>GSHMLDGCTPWPAEFAVRYREAGYWTGETFSDFVTDRTRRFADRLAVVGAGQRWTYAELGERSAVLATGLARLGIAAGDRVVVQLPNIPELFEVVFALFRLGALPVYALPAHRAHEITHLCTTAQAKALIIPDRHAGFDYRTMAAQLRHAGTAPEHVVVVGEPGGFTPLAELRADRPDPGVFTRPEASDAAFLQLSGGTTGLPKLIPRTHDDYLYSVRASAEICALGTDTVYLAALPAVHNFPM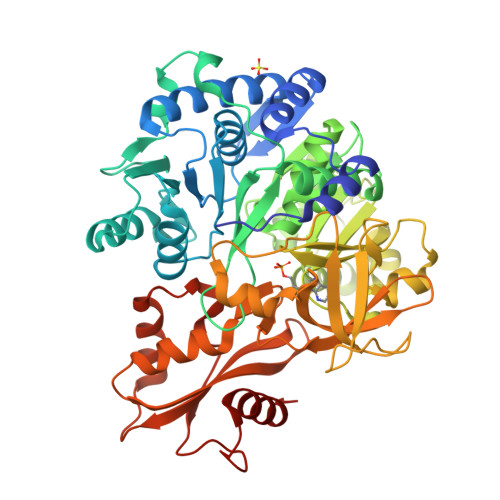SSPGFLGTFHAGGTVVLAPNPSPDTAFSLIETERVTITAVVPPIALQWLDAVEHGSQSHRDLSSLRVLQVGGAKFAPEAARRVRPVLGCTLQQVFGMAEGLVNYTRLDDPDDIITTTQGRPISPDDEIRIVDEADRPVPDGEVGHLLTRGPYTIRGYYRAEEHNATAFTPDGFYRTGDLVRRTPTGHLVVEGRAKDQINRGGEKVSAEEVENHILAHPAVHDAAVVGMSDPYLGERVCAYVIARTEPPSRSELLRFLRERGLASYKIPDRVEFVDRFPVTGVGKISRSELRRELARRLDTTR[2x]> MVATLFIADLHLQ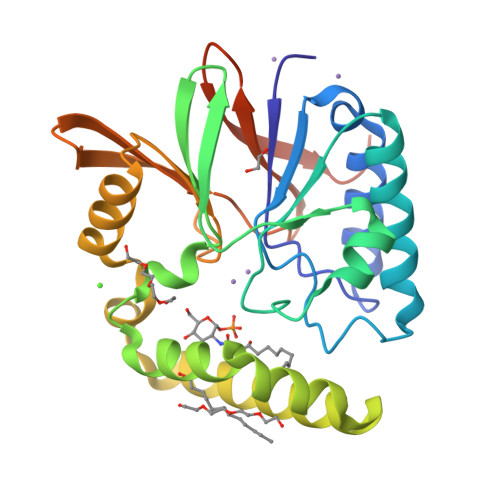TEEPAITAGFLRFLQGEARQADALYILGDLFEAWIGDDDPNPLHQQIASAIKAVVDAGVPCYFIHGNRDFLVGQRFARQSGMILLAEEERLDLYGREVLIMHGDTLCTDDQGYLAFRAKVHTPWIQRLFLALPLFIRHRIAARMRADSKAANSSKSMEIMDVNPQAVVDAMERHHVQWLIHGHTHRPAVHELQANGQPAWRVVLGAWHSEGSMVKVTPDDVELIHFPFLEENLYFQSHHHHHHHHHH> FNYDQPYRGQYHFSPQKNWMNDPNGLLYHNGTYHLFFQYNPGGIEWGNISWGHAISEDLTHWEEKPVALLARGFGSDVTEMYFSGSAVADVNNTS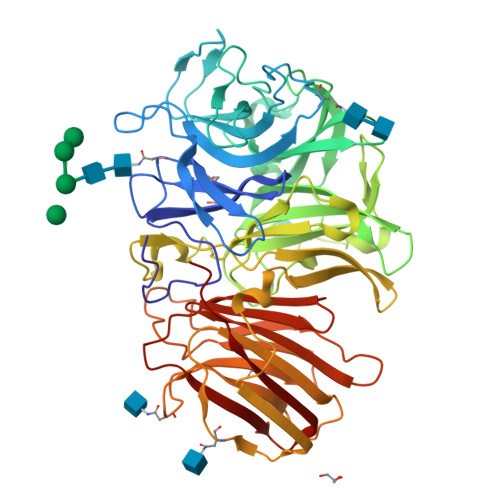GFGKDGKTPLVAMYTSYYPVAQTLPSGQTVQEDQQSQSIAYSLDDGLTWTTYDAANPVIPNPPSPYEAEYQNFRDPFVFWHDESQKWVVVTSIAELHKLAIYTSDNLKDWKLVSEFGPYNAQGGVWECPGLVKLPLDSGNSTKWVITSGLNPGGPPGTVGSGTQYFVGEFDGTTFTPDADTVYPGNSTANWMDWGPDFYAAAGYNGLSLNDHVHIGWMNNWQYGANIPTYPWRSAMAIPRHMALKTIGSKATLVQQPQEAWSSISNKRPIYSRTFKTLSEGSTNTTTTGETFKVDLSFSAKSKASTFAIALRASANFTEQTLVGYDFAKQQIFLDRTHSGDVSFDETFASVYHGPLTPDSTGVVKLSIFVDRSSVEVFGGQGETTLTAQIFPSSDAVHARLASTGGTTEDVRADIYKIASTWN> MAPPMTLQQWIIWKK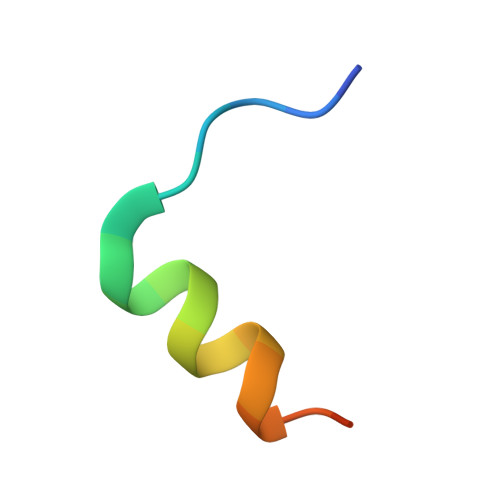MNKAH>[4x]MSNAEKALGVALIGTGFMGKCHAMAWRNVATAFGGLPPRLEVLADMPADKAHSLASSFGFARGTADWREAVSDPAVDVVSITTPNGLHREMAEAALAAGKHVWLEKPMALSVEDAQAMEAAARASDRRTIIGYN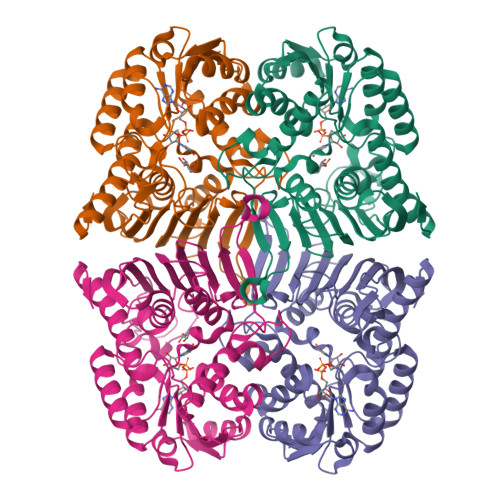YTRSPAFRAAVDLIAEGAIGRPIHFRGMYDEDYMADPDLPWSWRLTRKDGGLGALGDLGCHLVSVMVSLMGPVARVYAQADTVITDRPHQGGTARVENEDQAQALIRFASGTSGEFSCSRVARGYRCRLAWEVQGTEGTLRFDQERMNELWLYQPGRPEIDGFRRILTGPAQPGFAAFCPGGGHNFGFNEQKVVEAEMLRQAIAGRGKAWPDFTDGLTIERVIHGMATSAQTGQPVNFLEHHHHHH ARGININOSUCCINATE 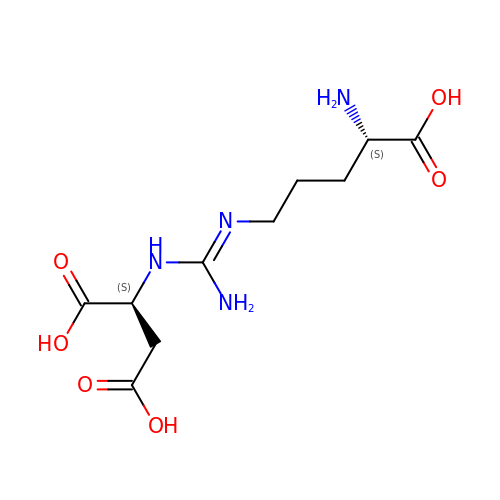| C10 H18 N4 O6 | KDZOASGQNOPSCU-WDSKDSINSA-N>SKKTVEFVDYVNPLMGTESTFAFSHGNTYPAVAVPWGMNFWSPQTGEN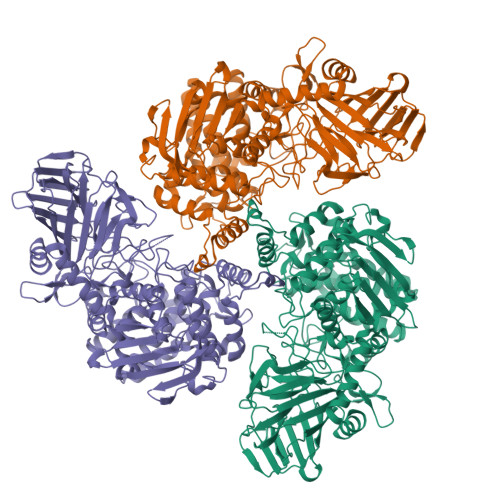GSGWMYTYTDSLMRGFRQTHQPSPWINDYGTFSIMPLAGELKMSHKERLVPFSHQQEKATPYNYSVTFNNGLQTSLSATSRGAVFEVSFPEKEDQYVVVDAYNGGSSITIEPEKRLVKGATRYNNGGVPDNFANYFMMEFSHPVIEYGTYNGDTLLHHQTDVAADYTCAYLKFDVPAGEKLTIRTASSFISPEQAAINFNREVADADVQLISGKAREQWNNYLGRVEAEGGTDEQLRTFYSCLYRTLLFPREFYEFDSQGNPVYYSPYDGNVHDGYMYTDNGFWDTFRAVHPLFTLLYPEVSERVTQSIINAYNESGFMPEWASPGHRGCMIGNNSVSLLVDAWMKGIQTVDAEKALEAMIHQTQARHAEIASVGRDGFEYYDKLGYVPYPEVPEATAKTLEYAYADWCIARFAESLGKQDIADQYYQKAPNYRNLYYPEHGFMWTKDAKGNWRDRFDATEWGGPFTEGSSWHWTWSVFHDPEGLSELMGGHEPMIARLDSMFVAPNTYNYGTYGFVIHEIAEMVALNMGQYAHGNQPVQHAIYLYDYIGQPWKTQYHLRNVMDKLYNSGSKGYCGDEDNGQTSAWYVFSAMGFYPVCPGMPEYAIGSPLFKKVTLHLPEGKNFVVSAADNAADRPYIRKALLNGQEFTRNYLTHDELKQGGELNLSMDSVPNQQRGTQPADFPYSYSK[3x]> GHMNSCSMPLGMESKAISDAQITASSYFTNMFATWSPSKARLHLQGRSNAWRPQVNNPKEWLQVDFQKTMKVTGVTTQGVKSAATSMYVKEFLISSSQDGHQWTLFFQNGKVKVFQGNQDSFTPVVNSLDPPLLTRYLR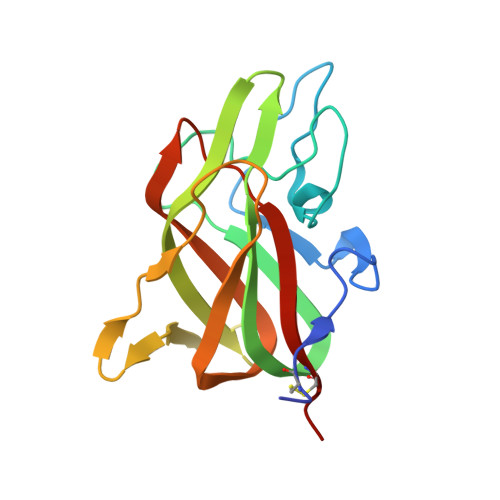IHPQSWVHQIALRMEVLGCEAQDLY>ANSHHHHHHGKLTSDFDNP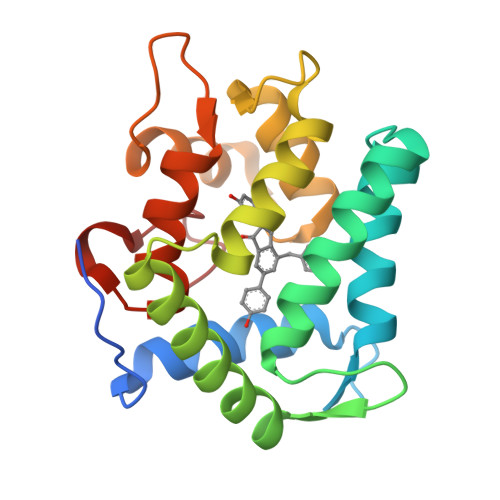RWIGRHKHMFNFLDVNHNGKISLDEMVYKASDIVINNLGATPEQAKRHKDAVEAFFGGAGMKYGVETDWPAYIEGWKKLATDELEKYAKNEPTLIRIWGDALFDIVDKDQNGAITLDEWKAYTKAAGIIQSSEDCEETFRVCDIDESGQLDVDEMTRQHLGFWYTMDPACEKLYGGAVP[16x]>SRRVASPSSELRRALEANEFIPYYQPLSPGQGGRWIGVEVLMRWRHPREGLIRPDLFIPFAERSGLIVPMTRALMRQVAEDLGGHAGKLE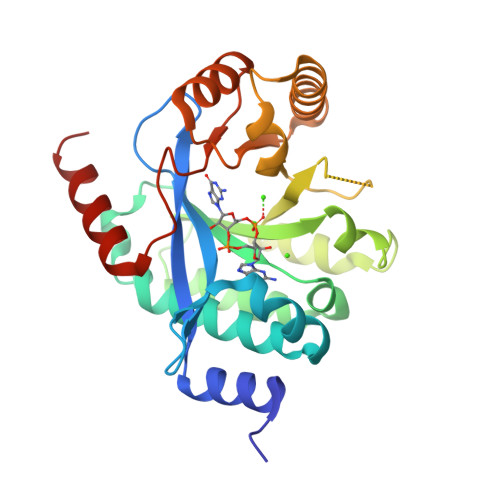PGFHIGFNISATHCHELALVDDCRELLAAFPPGHITLVLELTERELIESSEVTDRLFDELHALGVKIAIDDFGTGHSSLAYLRKFQVDCLKIDQSFVARIGIDTLSGHILDSIVELSAKLDLDIVAEGVETPEQRDYLAARGVDYLQGYLIGRPMPLESLLSSLTVQEGQGAS[2x]> MALRADQVSLIGQVFESYLLQHHRDDILGILRQGDDEAHYPVLVDALTLFETNMEIGEYFNAFPSQVLPIFDGALRRAAMAVLQAATPSPELRMKP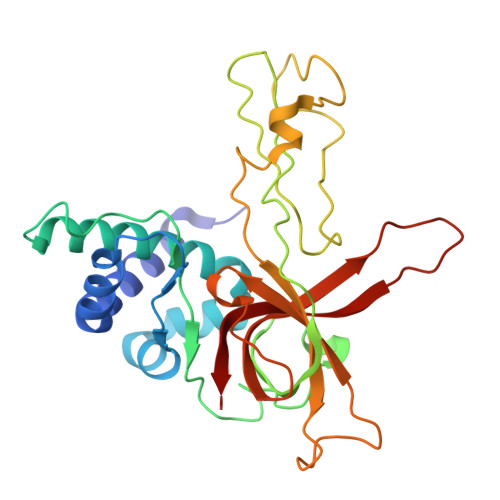NLHARISGLPICPELTREHIPKTRDVGHFLSVTGTVIRTSLVKVLEFERSYICNKCKHVFVAKADFEQYYAFCRPSACLNEEGCNSTKFTCLSGTSSSPSSCRDYQEIKIQEQVQRLSVGSIPRCMVVVLEDDLVDSCKSGDDITVYGVVMQRWKPFHQDARCDLELVLKANYVKVN> KPAEP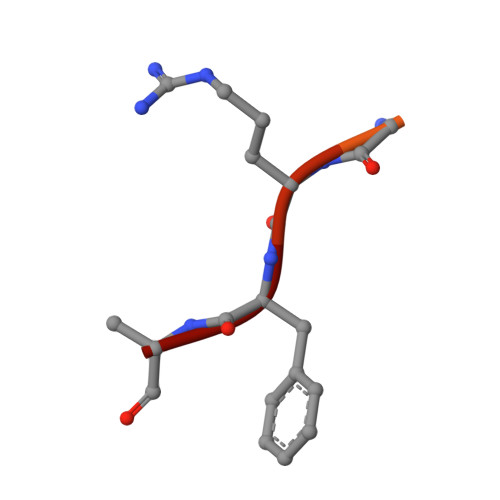QKTGRFA4-methoxy-6-phenyl-pyrimidin-2-amine | C11 H11 N3 O | 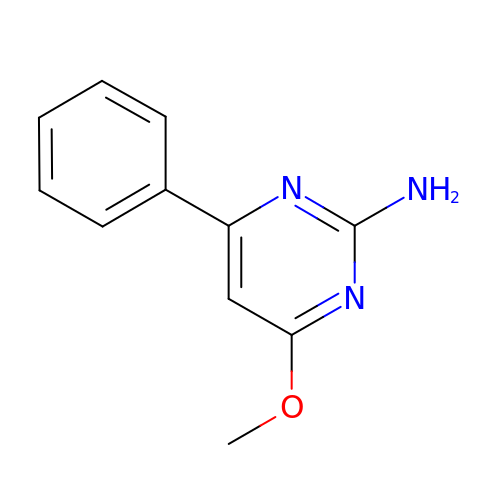NVXGRADJIFIBIO-UHFFFAOYSA-N> GAHMSYSYDAPSDFINFSSKQKNEESKKRQWALEDFEIGRPLGKGKFGNVYLAREKQSKFILALKVLFKAQLEKAGVEHQLRREVEIQSHLRHPNILRLYGYFHDATRVYLILEYAPLGTVYRELQKLSKFDEQRTATYITELANALSYVHSKRVIHRNIKPENLLLGSAGELKIADFGWSVHAPSSRRTTLCGTLDYLPPEMIEGRMHDEKVDLWSLGVLVYEFLVGKPPFEANTYQETYKRISRVEFTFPDFVTEGARDLISRLLKHNPSQRPMLREVLEHPW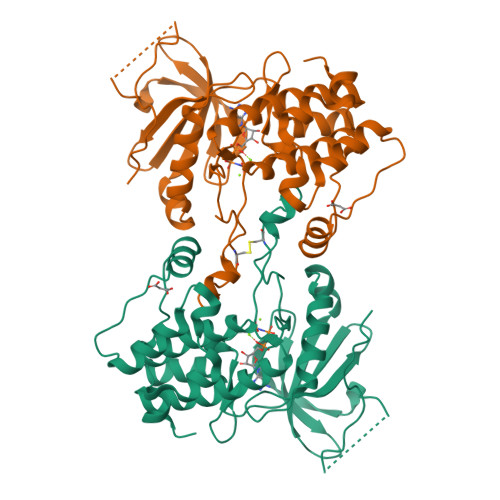ITANSSK> MGKRFSSFQAAQIRIARPTGQLDEIIRFYEEGLCLKRIGEFSQHNGYD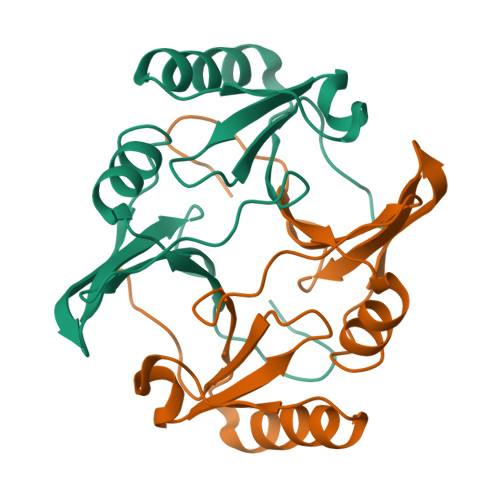GVMFGLPHADYHLEFTQYEGGSTAPVPHPDSLLVFYVPNAVELAAITSKLKHMGYQEVESENPYWSNGGVTIEDPDGWRIVFMNSKGISGK>[2x]MAKVLVLYYSMYGHIETMARAVAEGASKVDGAEVVVKRVPETMPPQL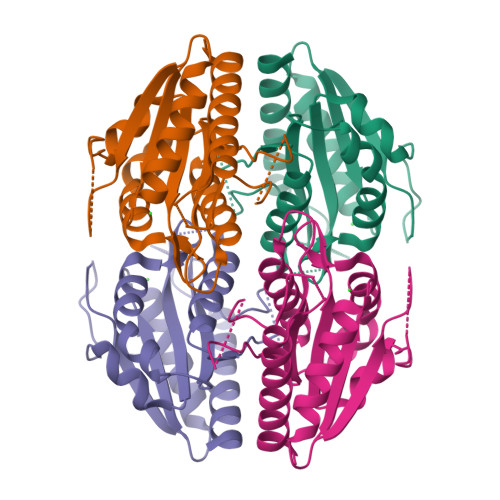FEKAGGKTQTAPVATPQELADYDAIIFGTPTRFGNMSGQMRTFLDQTGGLWASGALYGKLASVFSSTGTGGGQEQTITSTWTTLAHHGMVIVPIGYAAQELFDVSQVRGGTPYGATTIAGGDGSRQPSQEELSIARYQGEYVAGLAVKLNG>MAEMVETVCGPVPVEQLGKTLIHEHFLFGYPGFQGDVTRGTFREDESLRVAVEAAEKMKRHGIQTVVDPTPNDCGRNPAFLRRVAEETGLNIICATGYYYEGEGAPP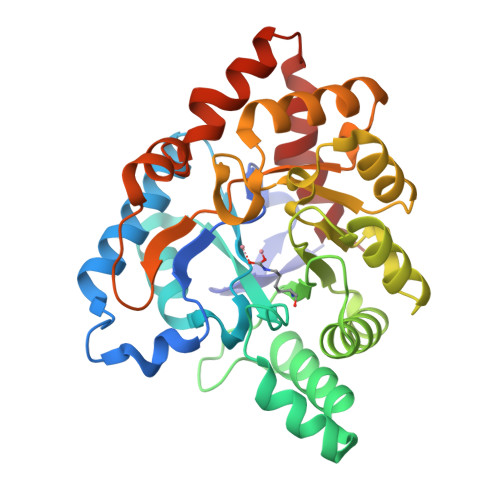YFQFRRLLGTAEDDIYDMFMAELTEGIADTGIKAGVIKLASSKGRITEYEKMFFRAAARAQKETGAVIITHTQEGTMGPEQAAYLLEHGADPKKIVIGHMCGNTDPDYHRKTLAYGVYIAFDRFGIQGMVGAPTDEERVRTLLALLRDGYEKQIMLSHDTVNVWLGRPFTLPEPFAEMMKNWHVEHLFVNIIPALKNEGIRDEVLEQMFIGNPAALFSA[2x]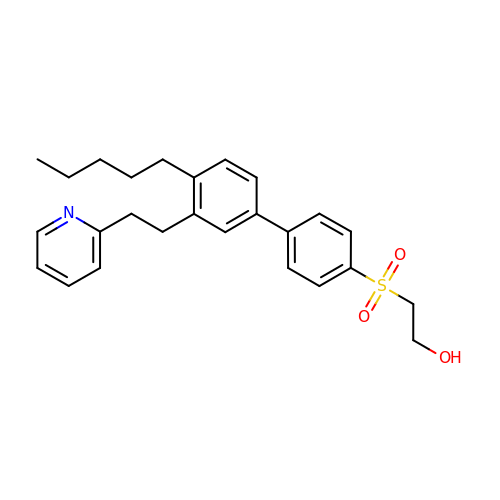2-({4'-pentyl-3'-[2-(pyridin-2-yl)ethyl][1,1'-biphenyl]-4-yl}sulfonyl)ethan-1-ol | C26 H31 N O3 S | XVDZECBAHSYSPZ-UHFFFAOYSA-N> DPTLEWFLSHCHIHKYPSKSTLIHQGEKAETLYYIVKGSVAVLIKDEEGKEMILSYLNQGDFIGELGLFEEGQERSAWVRAKTACEVAEISYKKFRQLIQVNPDILMRLSAQMARRLQVTSEKVGNLAFLDVTGRIAQTLLNLAKQP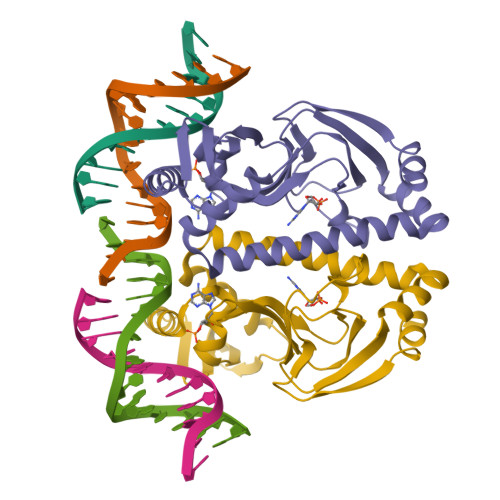DAMTHPDGMQIKITRQEIGQIVGCSRETVGRILKMLEDQNLISAHGKTIVVYG> MGSSHHHHHHSSGLVPRGSHMASSHAQTANWTEIYPGVWKATVGKPESYDLLKAAGAQPNKDALSKTEKVSFPFANGGVSLEVSGGKTYLRFPLQKEEQLYGFGLNFQTVHQRGKILELHVDHYGGKDSGRTHAPTPFYVSSNGYGVFINSARYIKVWAGTGVRKDSENFPTPKDRNTDKTWSSRPYSDAVEILVPAEGVEVYVFGGPKPIDAVKRYNLLNGGGYLPPRWGLGFTQRVMTRYTDKDVEKEVNDFKEKGYPLDFVGLEPGWQSKAYPGTFSWDKSRYPDPTSFVKKMKDQGIRLNLWINPYISPDAPFYKEIKPYTGSHTVWLGLVPDFTMAEARKPFFNQLLKDQIERGVSGYKIDEVDGYDYYLWPDAAKFPSGLSAEQMRQTYGLLVQRYSAELYKQRNERTFGLVRASNGGGTSFPYVIYNDYYNHQDFITALINSGFAGVLWTPEVRASKSGEEWLRRFQSNVFSPMAMINAWASGTKPWSYPEVEADVKKFALLRMQMMPYWYSAFARYHFEGMPPFRGMGLEEGFRQDAKVEKLNKVNLEENPYAEAASKEIKDQY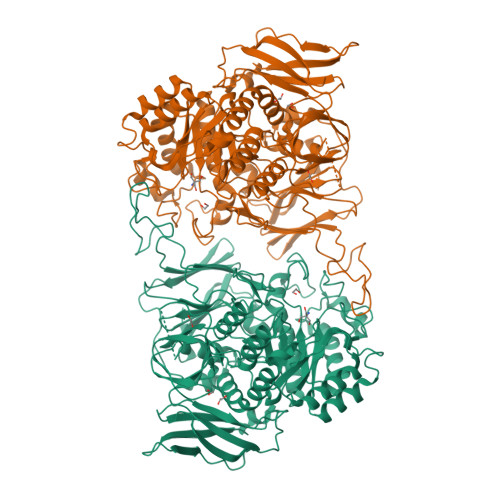MAGDDLLVAPMFAGEKSRKVVLPKGKWYDFYTGEYAGDGEVLDVTPGLDKIPVYVRDGGIVPMMPALLNSPKSNQKVDLEIRYYGNKPGEFKLYDDDGETFNYEKGDFSWRTIRVEKDKSGKVKGSISAAVKGKVNTVGKVTFTAMTK>[2x]HH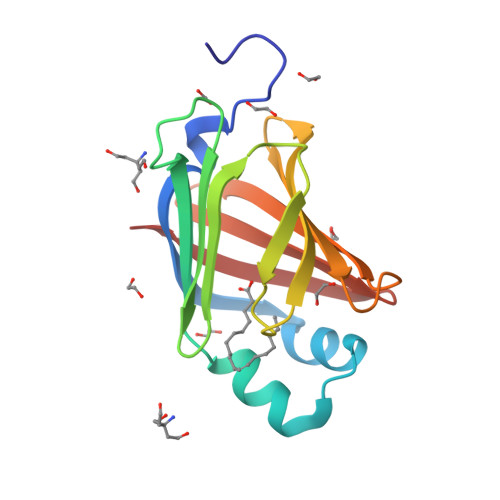HHGSKTLPDKFLGTFKLERDENFDEYLKARGYGWIMRQVIKLAGVTKKFRNAASGKPDRYDMENLTTKKDTHHKDWALGEEFQDEALDSTQHKITFDLKDPNTLTETHIKVDDPTDVETYEYRRDGDYLVMKMSWKGVSTSRYYKKQ>MLRIIDTETCGLQGGIVEIASVDVIDGKIVNPMSHLVRPDRPISPQAMAIHRITEAMVADKPWIEDVIPHYYGSEWYVAHNASFDRRVLPEMPGEWICTMKLARRLWPGIKYSNMALYKTRKLNVQTPPGLHHHRA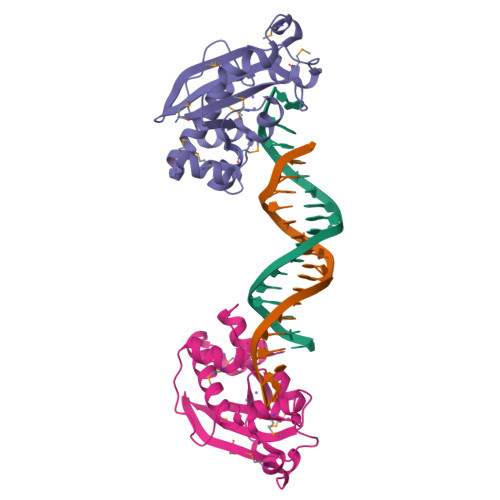LYDCYITAALLIDIMNTSGWTAEQMADITGRLEHHHHHH[2x]> TGEEVL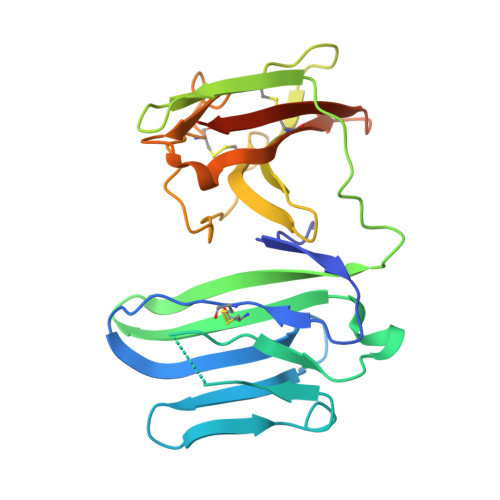WHTSVPFAENMSLECVYPSMGILTQVEWFKIGTQQDSIAIFSPTHGMVIRKPYAERVYFLNSTMASNNMTLFFRNASEDDVGYYSCSLYTYPQGTWQKVIQVVQSDSFEAAVPSNSHIVSEPGKNVTLTCQPQMTWPVQAVRWEKIQPRQIDLLTYCNLVHGRNFTSKFPRQIVSNCSHGRWSVIVIPDVTVSDSGLYRCYLQASAGENETFVMRLTVAEGKTDNQYTGTKHHHHHH>[2x]GPVHINKGGRPRQHLLSLTRRAQKHRLRELKIQVKEFADKEEGGDVKAVCLTLFLLALRARNEHRQADELEAIMQGRGSGLQPAVCLAIRVNTFLSCSQYHKMYRTVKAITGRQIFQPLHALRNAEKVLLPGYHPFEWQPPLKNVSSRTDVGIIDGLSGLASSVDEYPVDTIAKRFRYDSALVSALMDMEEDILEGMRSQDLDDYLNGPFTVVVKESCDGMGDVSEKHGSGPAVPEKAVRFSFTVMRITIEHGSQNVKVFEEPKPNSELCCKPLCLMLADESDHETLTAILSPLIAEREAMKSSELTLEMGGIPRTFKFIFRGTGYDEKLVREVEGLEASGSVYICTLCDTTRLEASQNLVFHSITRSHAENLQRYEVWRSNPYHESVEELRDRVKGVSAKPFIETVPSIDALHCDIGNAAEFYKIFQLEIGEVYKHPNASKEERKRWQATLDKHLRKRMNLKPIMRMNGNFARKLMTQETVDAVCELIPSEERHEALRELMDLYLKMKPVWRSSCPAKECPES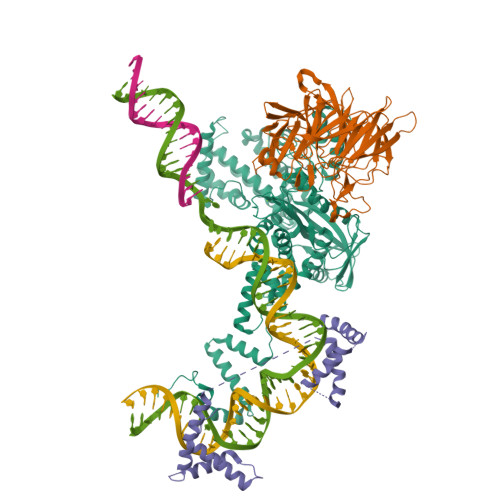LCQYSFNSQRFAELLSTKFKYRYEGKITNYFHKTLAHVPEIIERDGSIGAWASEGNESGNKLFRRFRKMNARQSKCYEMEDVLKHHWLYTSKYLQKFMNAHNA;>GPVSLQMVTVGHNIALIQPGFSLMNFDGQVFFFGQKGWPKRSCPTGVFHFDIKQNHLKLKPAIFSKDSCYLPPLRYPATCSYKGSIDSDKHQYIIHGGKTPNNELSDKIYIMSVACKNNKKVTFRCTEKDLVGDVPEPRYGHSIDVVYSRGKSMGVLFGGRSYMPSTQRTTEKWNSVADCLPHVFLIDFEFGCATSYILPELQDGLSFHVSIARNDTVYILGGHSLASNIRPANLYRIRVDLPLGTPAVNCTVLPGGISVSSAILTQTNNDEFVIVGGYQLENQKRMVCSLVSLGDNTIEISEMETPDWTSDIKHSKIWFGSNMGNGTIFLGIPGDNKQAMSEAFYFYTLRCSEEDLSEDQKIVSNSQTSTEDPGDSTPFEDSEEFCFS[2x];> MGKGDPKKPRGKMSSYAFFVQTCREEHKKKHPDASVNFSEFSKKCSERWKTMSAKEKGKFEDMAKADKARYEREMKTYIPPKGETKKKFKDPNAPKRPPSAFFLFCSEYRPKIKGEHPGLSIGDVAKKLGEMWNNTAADDKQPYEKKAAKLKEKYEKDIAAYR> GPLGSETQAGIKEEIRRQEFLLNSLHRDL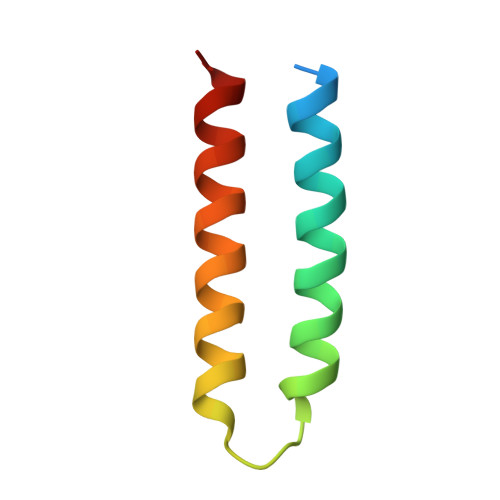QGGIKDLSKEHRLWEVLRILTALRRKLREA> MLANENSLLTMFRELGSGKLPLQIEQFERGKTIFFPGDPAERVYLLVK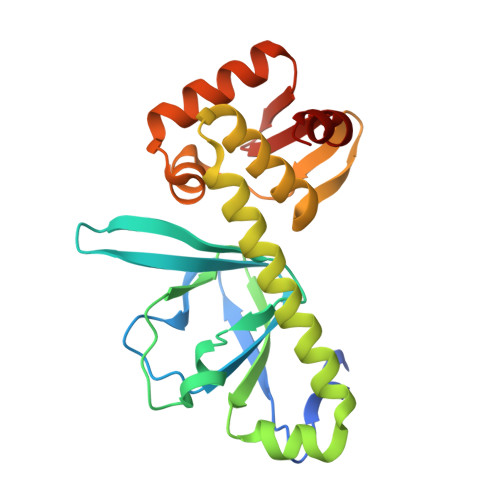GAVKLSRVYESGEEITVALLRENSVFGVLSLLTGQRSDRFYHAVAFTPVQLFSVPIEFMQKALIERPELANVMLQGLSSRILQTEMMIETLAHRDMGSRLVSFLLILCRDFGIPSPDGITIDLKLSHQAIAEAIGSTRVTVTRLLGDLRESKLIAIHKKRITVFNPVALSQQFS> MSEFNETKFSNNGTFFETEEPIVETKSISVYTPLI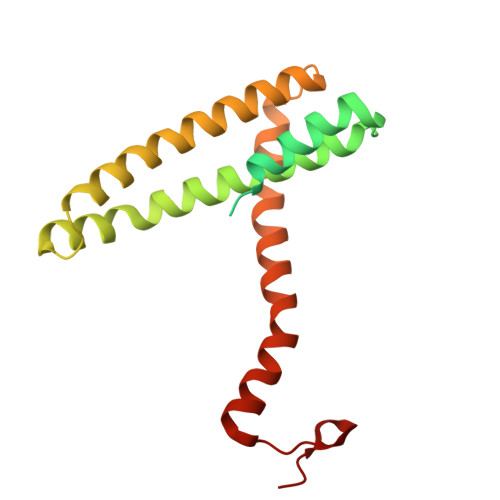YVFILVVSLVMFASSYRKKQAKKISEQPSIFDENDAHDLYFQIKEMSENEKIHEKVLKAALLNRGAESVRRSLKLKELAPQINLLYKNGSIGEDYWKRFETEVKLIELEFKDTLQEAERLQPGWVQLFVMVCKEICFNQALSRRYQSILKRKEVCIKEWELKINNDGRLVN> 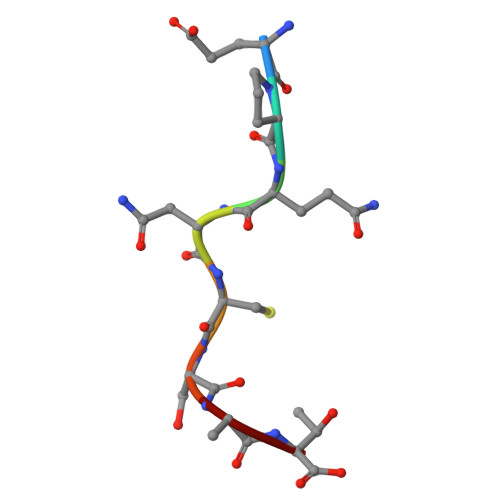EPQNCSAT> ITGQAACPESWIGFQRKCFYFSDDTKNWTSSQRFCDSQDADLAQVESFQEL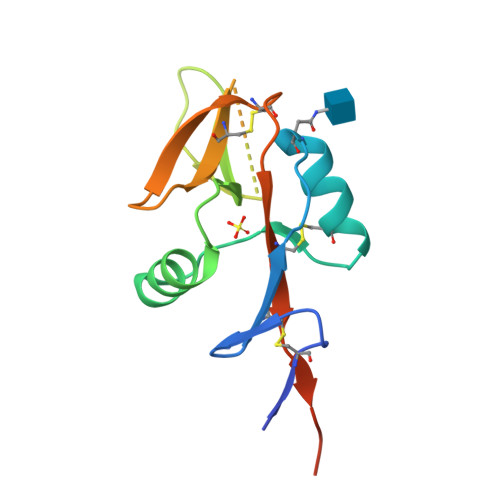NFLLRYKGPSDHWIGLSREQGQPWKWINGTEWTRQFPILGAGECAYLNDKGASSARCYTERKWICSKSDIHVGTKHHHHHHHHG> ALLQVTISLSKVELSVGESKFFTCTAIGEPESIDWYNPQGEKIISTQRVVVQKEGVRSRLTIYNANIEDAGIYRCQATDAKGQTQEATVVLEIYQKLTFREVVSPQEFKQGEDA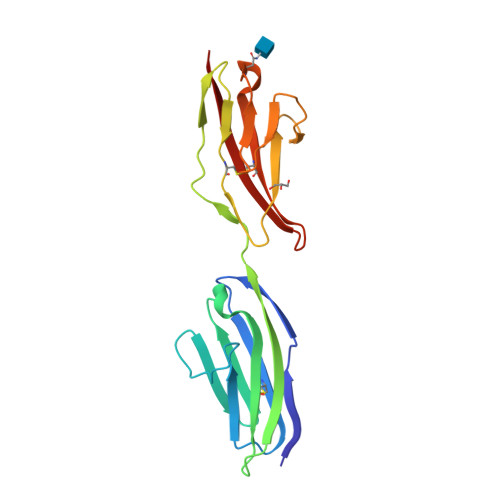EVVCRVSSSPAPAVSWLYHNEEVTTISDNRFAMLANNNLQILNINKSDEGIYRCEGRVEARGEIDFRDIIVIVNV>[2x]MHKVSATLLIIDDDEVVRESLAAYLEDSNFKVLQALNGLQGLQIFESEQPDLVICDLRMPQIDGLELIRRIRQTASETPIIVLSGAGVMSDAVEALRLGAADYLIKPLEDLAVLEHSVRRALDRAYLRVENQRYRDKLEAANRELQASLNLLQEDQNAGRQVQMNML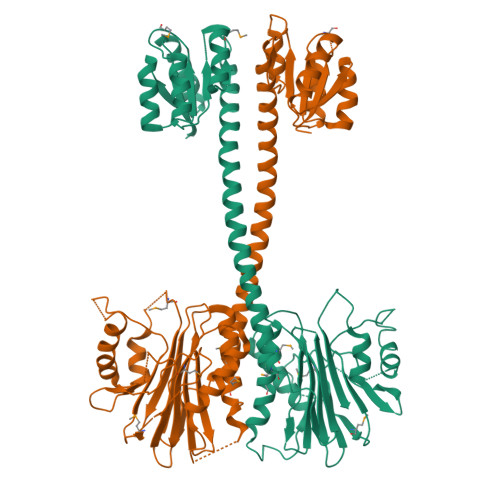PVTPWSIEGLEFSHRIIPSLYLSGDFVDYFRVDERRVAFYLADVSGHGASSAFVTVLLKFMTTRLLYESRRNGTLPEFKPSEVLAHINRGLINTKLGKHVTMLGGVIDLEKNSLTYSIGGHLPLPVLFVEGQAGYLEGRGLPVGLFDDATYDDRVMELPPSFSLSLFSDGILDVLPGATLKEKEASLPEQVAAAGGTLDGLRQVFGLANLAEMPDDIALLVLSRNLA> GAAQRQRALAIMCRVYVGSIYYELGEDTIRQAFAPFGPIKSIDMSWDSVTMKHKGFAFVEYEVPEAAQLALEQMNSVMLGGRNIKVGRPSNIGQAQP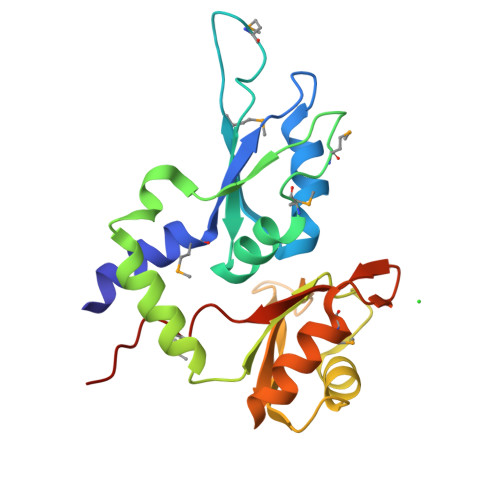IIDQLAEEARAFNRIYVASVHQDLSDDDIKSVFEAFGKIKSCTLARDPTTGKHKGYGFIEYEKAQSSQDAVSSMNLFDLGGQYLRVGKAVTPPMPLLTPATPG>SNAMRNYIQGIDHVQVAAPVGCEEEARAFYGETIGME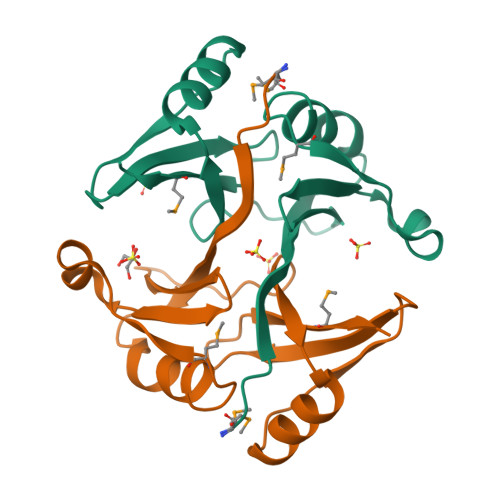EIPKPEELKKRGGCWFKCGNQEIHIGVEQNFNPAKRAHPAFYVLKIDEFKQELIKQGIEVIDDHARPDVIRFYVSDPFGNRIEFMENKN[2x]> TKSVKRGVAYDVASPADLSALSTGMSWWYNWSPKPHDRLAAYDYAGQYNVDFVPMVWNANLDDGQLKLYLLAHPGIRYLLVINEPNLVDQANMTPQAAAQLWPRLEQISAQTGVKLVGPAMNWGTMTGYGDPVAWLDAFYAAYASAHQGRDPQIDYLAFHWYDYGLSSMLDRLSRYGKPFWVTEFANWHTLDDGLQIDSLEKQKQQMAEMVTMLERRSDVFRYAWFTGRMTPDPHFSSLLDAEGRLTELG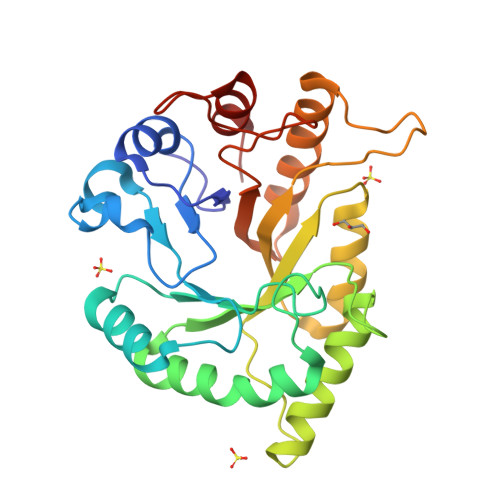QYYLSLPYS>[2x]MTLGTNQVSKTHSFMTVSLIELWERFGYYGMQALIVYFMVQRLGFDDSRANLVWSACAALIYVSPAIGGWVGDKILGTKRTMLLGAGILSVGYALMTVPTENTWFMFSALGVIVVGNGLFKPNAGNLVRKIYEGDDSKIDSAFTIYYMAVNVGSTFSMLLTPWIKDYVNAQYGNEFGWHAAFAVCCVGILVGLGNYALMHKSLANYGSEPDTRPVNKKSLAIVLALAALSVVASAIILEYEDVARVFVYAAGVAVLGIFFHLIRTSEPSERAGLIAALILTVQTVFFFIFYQQMSTSLALF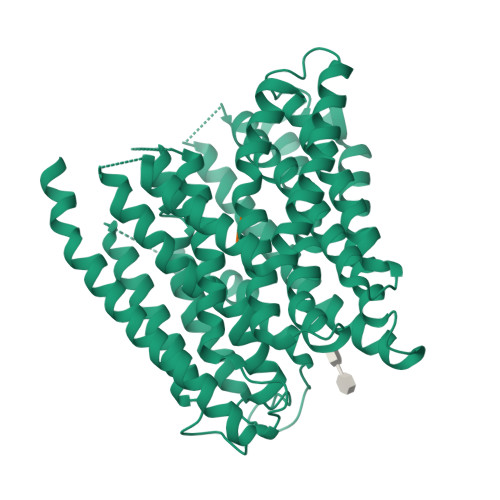ALRNVDWDFQVFGTHLWTWSPAQFQALNPIWIMVLSPVLAWSYSWAGRNNKDFSIAAKFALGFAVVAIGFFIYGFAGQFAVNGKTSSWVMIWGYASYSLGELLVSGLGLAMIARYVPARMGGFMMGAYFVASGISQYLGGVVANFASVPQDLVDPLQTLPVYTNLFNKLGVAAVVCTIIALAVLPLMRRLTESHHAHSSIENNAAASLRDVKAEQAENLYFQ;>[2x]AAA>MAEKPKLHYSNIRGRMESIRWLLAAAGVEFEEKFIKSAEDLDKLRNDGYLMFQQVPMVEIDGMKLVQTRAILNYIASKYNLYGKDIKEKALIDMYIEGIADLGEMILLLPFTQPEEQDAKLALIQEKTKNRYFPAFEKVLKSHGQDYLVGNKLSRADIHLVELLYYVEELDSSLISSFPLLKALKTRISNLPTVKKFLQPGSPRKPPMDEKSLEESRKIFRF[8x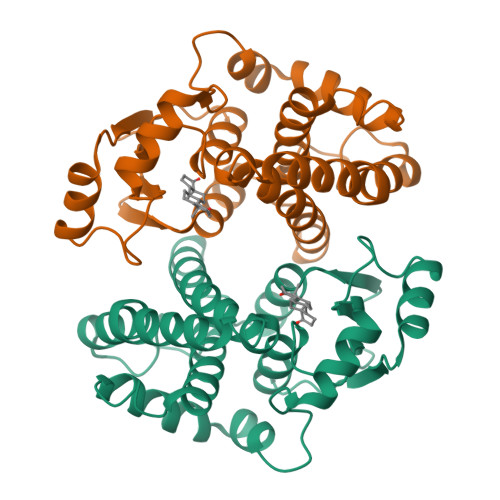]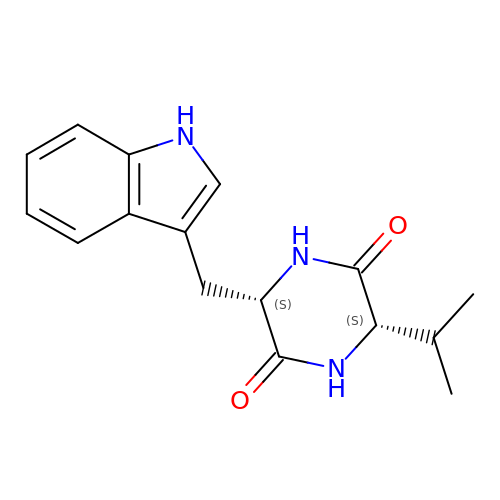(3S,6S)-3-[(1H-indol-3-yl)methyl]-6-(propan-2-yl)piperazine-2,5-dione | C16 H19 N3 O2 | WNWCQIPRIITCPM-KBPBESRZSA-N> KETCSTGLYTHSGECCKACNLGEGVAQPCGANQTVCEPCLDNVTFSDVVSATEPCKPCTECLGLQ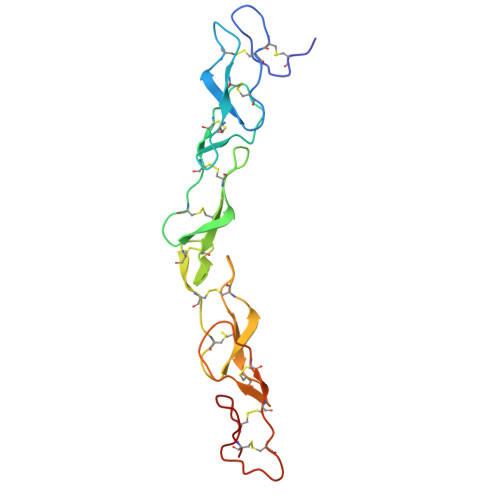SMSAPCVEADDAVCRCAYGYYQDEETGHCEACSVCEVGSGLVFSCQDKQNTVCEECPEGTYSDEANHVDPCLPCTVCEDTERQLRECTPWADAECE>SLGLQDFDLLRVIGRGSYAKVLLVRLKKTDRIYAMKVVKKELVNDDEDIDWVQTEKHVFEQASNHPFLVG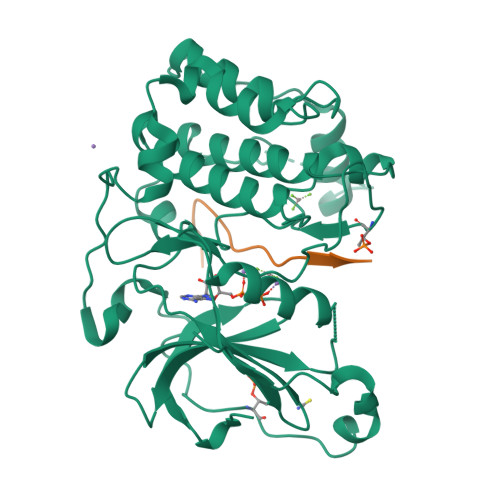LHSCFQTESRLFFVIEYVNGGDLMFHMQRQRKLPEEHARFYSAEISLALNYLHERGIIYRDLKLDNVLLDSEGHIKLTDYGMCKEGLRPGDTTSTFCGTPNYIAPEILRGEDYGFSVDWWALGVLMFEMMAGRSPFDIVGSSDNPDQNTEDYLFQVILEKQIRIPRSLSVKAASVLKSFLNKDPKERLGCHPQTGFADIQGHPFFRNVDWDMMEQKQVVPPFKPNISGEFGLDNFDSQFTNEPVQLTPDDDDIVRKIDQSEFEGFEYINPLLMSAEECV[2x];>[2x]ERMRPFKRQGSVRRRV> MFFELEDIKRRHSLYWDIYNVQGWVRRPDSTLYNNVKRGVTAGVVASLVQENITALVENCKLLATKYEKPQNLRQAATFMKEVFKLENYRKAVWNRSQYALCIGTFDIGARLATFRWLNNGWQRVFAGFEFNFVRKIPTTMLAALFTAPFSVPFELARMAYYGDKTFPKELQRGYSSYLSALARIPFEEGPYFLFKNSFPLIIRNFFQT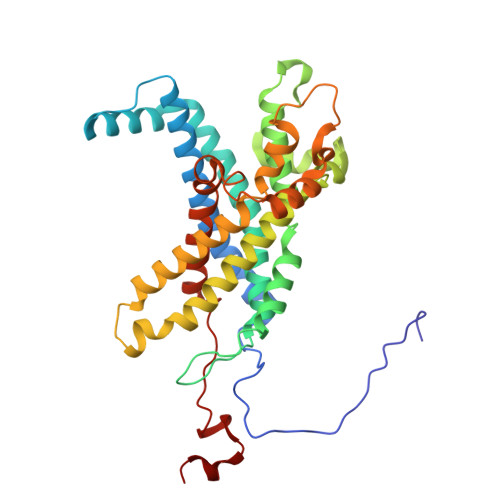FTLFYTYDFLKDKASFAWRVGEQNEYACKMIIAGISTYLAAVFSYPWMVTREMVDFWPKVPGAPCTFNGNYRKAAVWIWYHEFSGNYFAGFFTKYFWKASPGMFLTLMLADKVGLFDQTTVDNFGGAGNNSWEDTFV>APQQINDIVHRTITPLIEQQKIPGMAVAVIYQGKPYYFTWGYADIAKKQPVTQQTLFELGSVSKTFTGVLGGDAIARGEIKLSDPTTKYWPELTAKQWNGITLLHLATYTAGGLPLQVPDEVKSSSDLLRFYQNWQPAWAPGTQRLYANSSIGLFGALAVKPSGLSFEQAMQTRVFQPLKLNHTWINVPPAEEKNYAWGYREGKAVHVSPGALDAKAYGVKSTIEDMARWVQSNLKPLDINEKTLQQGIQLAQSRYWQTGDMYQGLGWEMLDWPVNPDSIINGSDNKIALAARPVKAITPPTPAVRASWV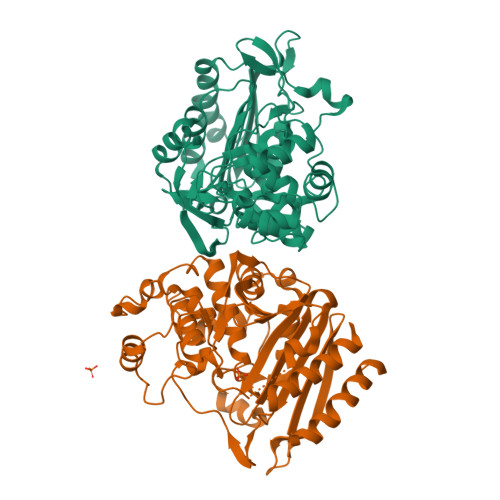HKTGATGGFGSYVAFIPEKELGIVMLANKNYPNPARVDAAWQILNALQ[2x]> DTIKWVTLKHNGVIFPPPYQPLPSHIKLYYDGKPVDLPPQAEEVAGFFAALLESDHAKNPVFQKNFFNDFLQVLKESGGPLNGIEIKEFSRCDFTKMFDYFQLQKEQKKQLTSQEKKQIRLEREKFEEDYKFCELDGRREQVGNFKVEPPDLFRGRGAHPKTGKLKRRVNPED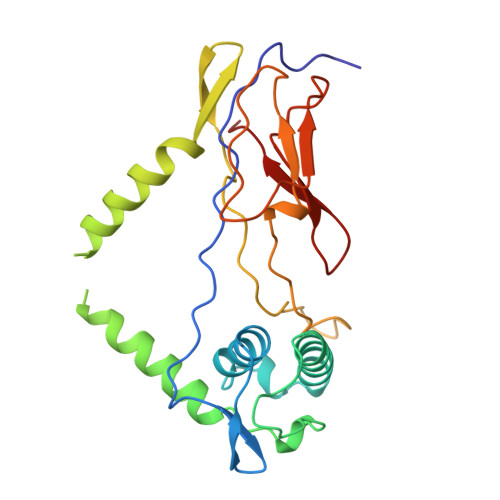IVLNLSKDAPVPPAPEGHKWGEIRHDNTVQWLAMWRENIFNSFKYVRLAA(2R)-4-[4-fluoro-2-(trifluoromethyl)phenyl]-2-methyl-1-{[3-(1H-1,2,4-triazol-1-yl)phenyl]sulfonyl}piperazine 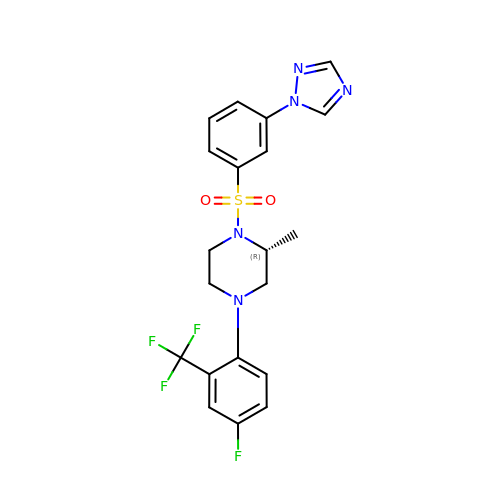| C20 H19 F4 N5 O2 S | ALJLAOVBUJZEDK-CQSZACIVSA-N4-(4-{[(2-chlorophenyl)carbamoyl]amino}-1H-pyrazol-1-yl)-N-(oxetan-3-yl)thiophene-2-carboxamide 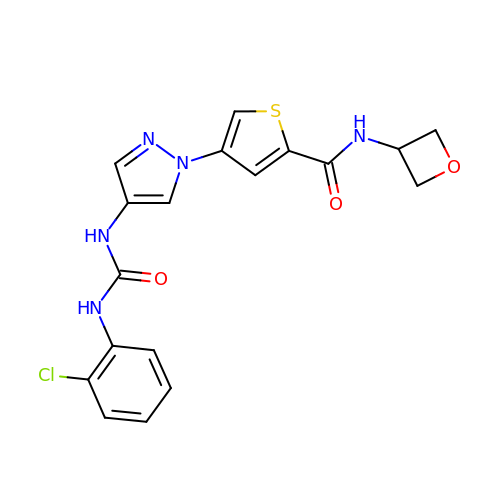| C18 H16 Cl N5 O3 S | FPVKFPPNOMNINZ-UHFFFAOYSA-N>[4x]RYRGSKWAGKKSIPAFIDNDYNEADQVIENLQRNELTPREIADFIGRELAKGKKKGDIAKEIGKSP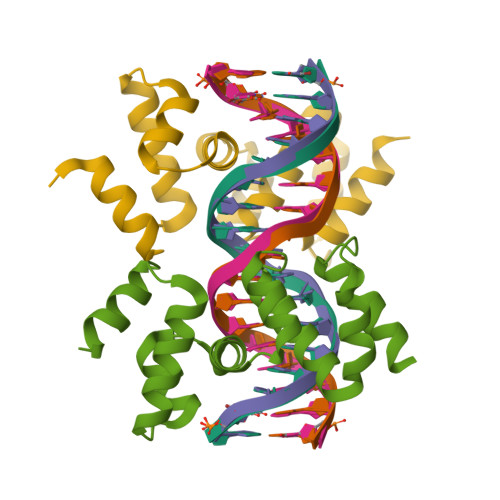AFITQHVTLLDLPEKIADAFNTGRVRDVTVVNELVTAFKKRPEEVEAWLDDDTQEITRGTVKLLREFLDEKGRDPNTVDAFNGQTDAERDAEAGDGQDGEDGDQDGKDAKEK>SNAIRPTIGQQMETGDQRFGDLVFRQLAPNVWQHTSYLDMPGFGAVASNGLIVRDGGRVLVVDTAWTDDQTAQILNWIKQEINLPVALAVVTHAHQDKMGGMDALHAAGIATYANALSNQLAPQEGLVAAQHSLTFAANGWVEPATAPNFGPLKVFYPGPGHTSDNITVGIDGTDIAFGGCLIKDSKAKSLGNLGDADTEHYAASARAFGAAFPKASMIVMSHSAPDSRAAITH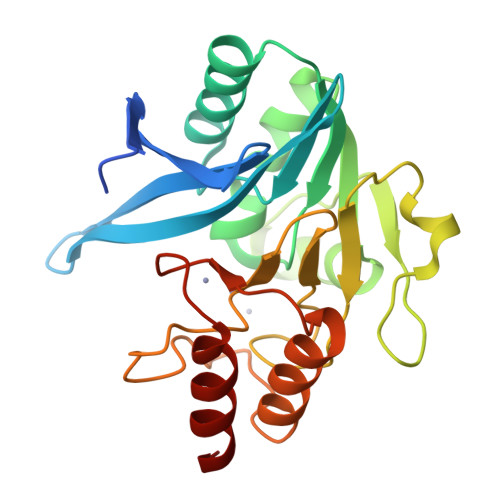TARMADKLR[2x]ethyl 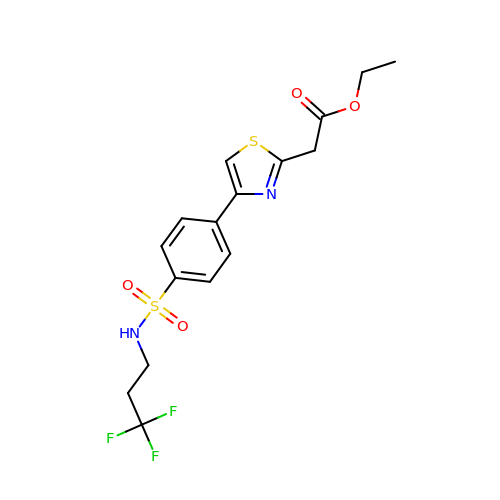2-[4-[4-[3,3,3-tris(fluoranyl)propylsulfamoyl]phenyl]-1,3-thiazol-2-yl]ethanoate | C16 H17 F3 N2 O4 S2 | BOOGQWHJJOHPJE-UHFFFAOYSA-N> MLSHAVPRLRLAAAAVKAAEWYAAENRRKQKGGDVIREKVDCTAPLWFDDTEQNLLAREQHVRSPAYRELHRPALTNAAMGLYGGEPGFEKAHRVWVDPDRPHIKHIYNQTALARNLRYARYGYFKRDMHLLDVDKLVRHARLLPTPGRLLTDFLYQRVPLPDKSCAALIRYQRQQIEMLEVWGRHASFQCAVEMFERMIVTNIPPVEVGVETHGEMVLCAAACGKWEEGWNVYANRARELEKESPESFILNTFFFDALLTLCVAAGRVSEGIDTLEEVIKRNLRPRGTMLNKAMILYSILGEQMSK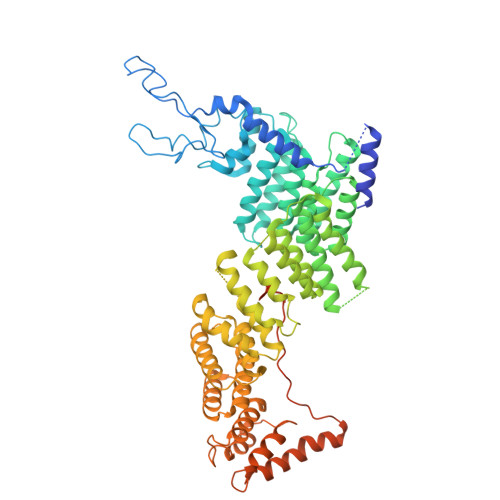HEASRATSEGERSYLCEPEEVEKMGLEVWSLFDFYQLPRTTASIEAYMRMCCAFNKPTLVLKAQGFADASDIRLSIECFHWLVYAIRGVAGFGDYVMDVLSQLRPRGLTPDFVLFTLSFMYCALQRDGELALAIFDQHFVHQNMNPTPEMVLLFIQACSNCEEPTAVMLERSETLIKRLEAVGSSVDLISPIYDQFLELCAHLGAVASGFSALKRIVGFGKPLTTRMINSLLLANSNAISSNGSLSMTEELVGFFTLLKIRPNADTEICVNLCRDAFGESPVVNDFIKVIGESLQGDSEKGEAPQYDEDIPVIQVPPHELRQLRTEWKLSPRDIVLRRFGQHTKPPGKAALDVGSMRGSVIPFGRSPGEQLV> GLIVDTRDVEERVHVMRKTKLAPTVAHGVFNPEFGPAALSNKDPRLNEGVVLDEVIFSKHKSDTKMSAEDKALFRRCAADYASRLHSVLGTANAPLSIYEAIKGVDGLDAMEPDTAPGLPWALQGKRRGALIDFENGTVGPEVEAALKLMEKREYKFACQTFLKDEIRPMEKVRAGKTRIVDVLPVEHILYTRMMIGRFCAQMHSNNGPQIGSAVGCNPDVDWQRFGTHFAQYRNVWDVDYSAFDANHCSDAMNIMFEEVFRTEFGFHPNAEWILKTLVNTEHAYENKRITVEGGIPSGCSATSIINTILNNIYVLYALRRHYEGVELDTYTMISYGDD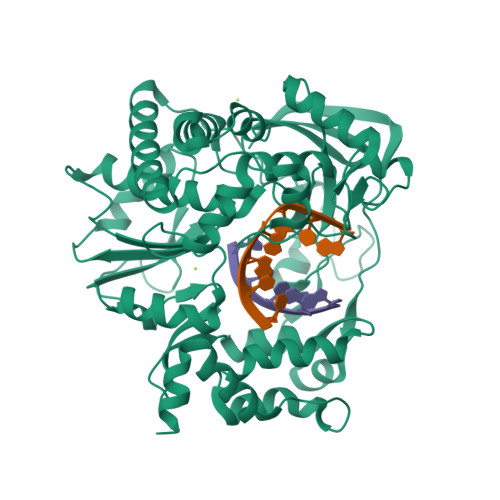IVVASDYDLDFEALKPHFKSLGQTITPADKSDKGFVLGHSITDVTFLKRHFHMDYGTGFYKPVMASKTLEAILSFARRGTIQEKLISVAGLAVHSGPDEYRRLFEPFQGLFEIPSYRSLYLRWVNAVCGDAAALEHH N-[4-(4-acetylpiperazin-1-yl)benzyl]-N-(2-methylpropyl)-1-phenylmethanesulfonamide 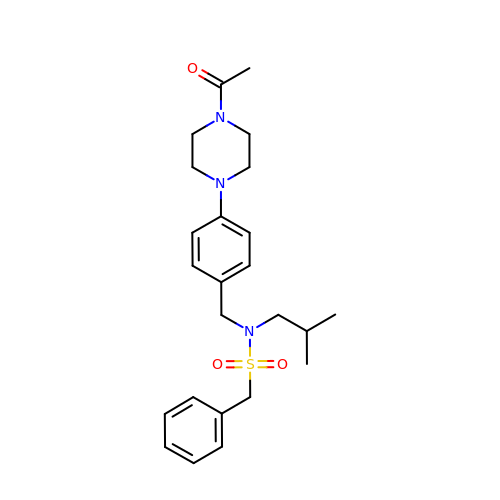| C24 H33 N3 O3 S | CYRKYCCPWKLCDV-UHFFFAOYSA-N> MTQFTQNTAMP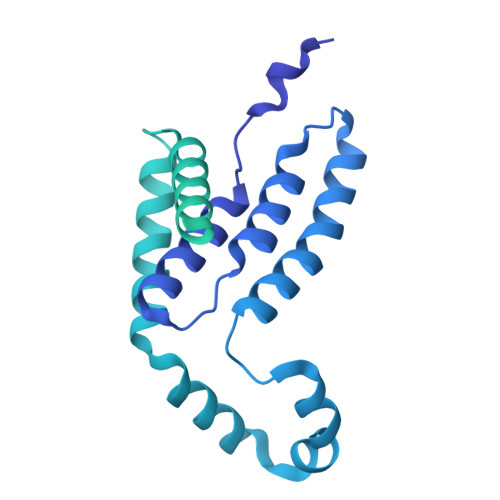SSLWQYWRGLSGWNFYFLVKFGLLWAGYLNFHPLLNLVFAAFLLMPLPRYSLHRLRHWIALPIGFALFWHDTWLPGPESIMSQGSQVAGFSTDYLIDLVTRFINWQMIGAIFVLLVAWLFLSQWIRITVFVVAILLWLNVLTLAGPSFSLWPAGQPTTTVTTTGGNAAATVAATGGAPVVGDMPAQTAPPTTANLNAWLNNFYNAEAKRKSTFPSSLPADAQPFELLVINICSLSWSDIEAAGLMSHPLWSHFDIEFKNFNSATSYSGPAAIRLLRASCGQTSHTNLYQPANNDCYLFDNLSKLGFTQHLMMGHNGQFGGFLKEVRENGGMQSELMDQTNLPVILLGFDGSPVYDDTAVLNRWLDVTEKDKNSRSATFYNTLPLHDGNHYPGVSKTADYKARAQKFFDELDAFFTELEKSGRKVMVVVVPEHGGALKGDRMQVSGLRDIPSPSITDVPVGVKFFGMKAPHQGAPIVIEQPSSFLAISDLVVRVLDGKIFTEDNVDWKKLTSGLHKQHRSPRTQMQ In this study, we show that GAS7 plays a critical role in phagocytic cup formation in macrophages. Crystallographic, electron microscopic, biochemical and cellular localization analyses revealed that the GAS7 F-BAR domain possesses unique hydrophilic loops that contribute to two-dimensional sheet formation of GAS7 on flat membranes of phagocytotic cup, indicating that the sheet-like assembly of GAS7 is essential for phagocytosis. In addition to the F-BAR domain, GAS7b possess a WW domain, and GAS7cb and GAS7c possesses a WW and an SH3 domain, while GAS7d contains only the F-BAR domain. The structures of the F-BAR domains in both crystals were almost identical, with a root mean square deviation of 1.2 Å. The GAS7 F-BAR domain forms a helical-bundle dimer with a shallow concave curvature, which is one of the flattest curvatures amongst the known F-BAR domains.

The asymmetric unit of the F-BAR domain crystal contained two F-BAR dimers. These dimers interacted with their symmetry-related dimers, forming filamentous oligomers with asymmetric flat surfaces, which we refer to as flat filamentous oligomers (FFOs). The two FFOs formed by the different dimers in the asymmetric unit were essentially identical to each other. The FFOs had a width of ~14 nm with a ~5 nm distance between adjacent F-BAR dimers, while the F-BAR dimers were ~22 nm in length. The lateral alignment of F-BAR domains in FFO appeared to be similar to the pitch of the GAS7 striations on the monolayered membrane. The FFOs of the F-BAR domain in the crystals appeared to be mediated by two GAS7-specific loops, filament forming loop 1 (FFL1)  (aa 171–197; GAS7cb amino-acid residue numbers) and filament forming loop 2 (FFL2) (aa 206–219), which are located on the convex and concave surfaces, respectively. The positions of the two FFL1s and FFL2s are symmetrical; however, one of the two FFL1s at the convex surface of the dimer interacted with the tip of the adjacent dimer, and one of the two FFL2s at the concave surface of the dimer interacted with a conserved region on the convex surface of the adjacent dimer in the FFO, thus tilting the helix bundle relative to the plane of the FFO. Due to asymmetry, one side of the flat surfaces of the FFO is more positively charged than the other. Thus, we supposed that this surface could be the membrane-binding surface. One of the two FFL2s lacks contacts with the adjacent dimer and protrudes from the FFO surface, suggesting the direct contact of the FFL2 with the membrane.

>[4x]MNHKVHHHHHHMELGTLEGSRKQSKENTITINCVTFPHPDTMPEQQLLKPTEWSYCDYFWADKKDPQGNGTVAGFELLLQKQLKGKQMQKEMSEFIRERIKIEEEYAKNLAKLSQNSLAAQEEGSLGEAWAQVKKSLADEAEVHLKFSAKLHSEVEKPLMNFRENFKKDMKKCDHHIADLRKQLASRYASVEKARKALTERQKDLEMKTQQLEIKLSNKTEEDIKKARRKSTQAGDDLMRCVDLYNQAQSKWFEEMVTTTLELERLEVERVEMIRQHLCQYTQLRHETDMFNQSTVEPVDQLLRKVDPAKDRELWVREHKTGNIRPVDMEI> SNRLDGKVAIITGGTLGIG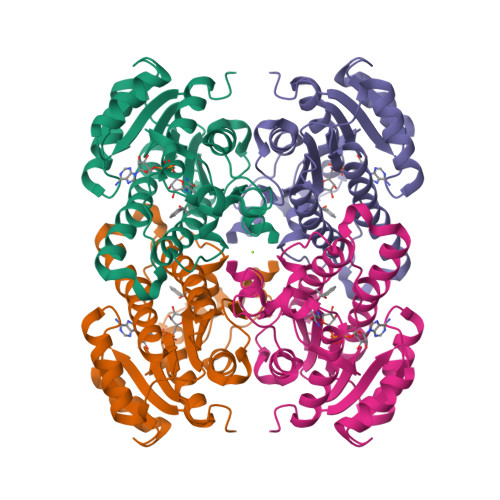LAIATKFVEEGAKVMITDRHSDVGEKAAKSVGTPDQIQFFQHDSSDEDGWTKLFDATEKAFGPVSTLVNNAGIAVNKSVEETTTAEWRKLLAVNLDGVFFGTRLGIQRMKNKGLGASIINMSSIEGFVGDPSLGAYNASKGAVRIMSKSAALDCALKDYDVRVNTVHPGYIKTPLVDDLPGAEEAMSQRTKTPMGHIGEPNDIAYICVYLASNESKFATGSEFVVDGGYTAQ> MAHHHHHHAEPLKIALVETLSGPQ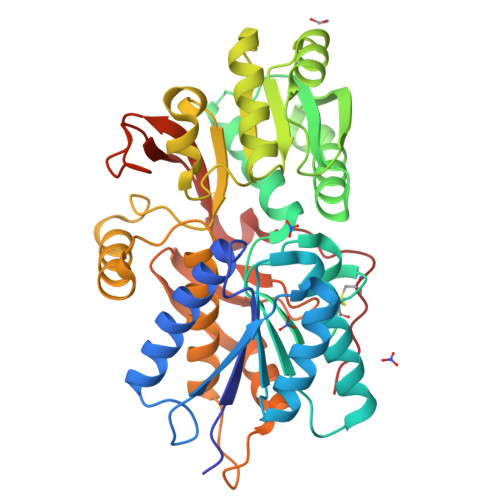ASTGLLYRAAVLYQLGKINEAGGFNGEKIQILEYDNQGGPVGAADRVKAAIADGAQIIVQGSSSAVAGQITEDVRKYNLRNKGKEVLYLNLGAEALELTGSKCHFYHFRFSPNAAIRFKTVAQGMKDKGILGERAYSINQNYSWGVDVENTVVANAKEIGYEVVDKTLHEVNKIQDFSPYVAKIQAANVDTVFTGNWSNDLLLLMKAASGAGLKAKFATSFLDQPGNIGNAGAIAEGHIVSTPFNPEANGEASMAFAEDYKKVTGHYPSYVEPAAVFGLQLFGEALKNVKPGEGKINTTDIALAIENASVKTPMGDYSMRSDDHQAKFPMVVQEVSKKARIKADGTEYGFLPFKTFTGDESIDPVQESCSMKRPG The solute carrier 13 (SLC13) family comprises electrogenic sodium ion–coupled anion cotransporters, segregating into sodium ion–sulfate cotransporters (NaSs) and sodium ion–di- and–tricarboxylate cotransporters (NaDCs). NaS1 and NaDC1 regulate sulfate homeostasis and oxidative metabolism, respectively. From an overall view, both the NaDC1 and NaS1 form a homodimer, and each protomer consists of 11 TMDs. The rest TMDs form the core domain that is responsible for substrate recognition and conformational change to complete the transport cycle.

In this study, we determined the cryo–electron microscopy structures of human NaS1, capturing inward-facing and combined inward-facing/outward-facing conformations within a dimer both in apo and sulfate-bound states. For clarity, we have designated the NaS1 conformations as “IN/IN” for the inward-facing state, “IN/OUT” for the combined inward-facing/outward-facing states within a dimer, and “OUT/OUT” for the outward-facing conformation of NaDC1. Furthermore, the NaS1_IN/OUT conformations imply that each protomer within the dimer can independently execute the substrate transport cycle within SLC13 members. In this context, it is remarkable that TM1 to TM3 and TM9 of the dimerization domain maintain its structural integrity throughout the conformational change process, only minor changes of TM4, TM7, and TM8 are detected, emphasizing its role as a stable scaffold. However, the core domain, a pivotal player in the conformational transition, undergoes a notable movement. Furthermore, a more intricate conformational landscape emerges upon comparing the IN subunits of NaS1-IN/IN with the OUT subunits of NaS1_IN/OUT. This analysis reveals a dual-layered transition involving both horizontal and vertical displacements. Notably, the N and C halves within a given subunit undergo a remarkable conformational interchange, a dynamic interplay that mirrors the broader conformational shift of NaS1 during the transport cycle. Specifically, the binding pocket in the outward facing conformation of NaS1 could not accommodate the cholesterol molecule.

>MADYKDDDDKSGRMKFFSYILVYRRFLFVVFTVLVLLPLPIVLHTKEAECAYTLFVVATFWLTEALPLSVTALLPSLMLPMFGIMPSKKVASAYFKDFHLLLIGVICLATSIEKWNLHKRIALKMVMMVGVNPAWLTLGFMSSTAFLSMWLSNTSTAAMVMPIAEAVVQQIINAEAEVEATQMTYFNGSTNHGLEIDESVNGHEINERKEKTKPVPGYNNDTGKISSKVELEKNSGMRTKYRTKKGHVTRKLTCLCIAYSSTIGGLTTITGTSTNLIFAEYFNTRYPDCRCLNFGSWFTFSFPAALIILLLSWIWLQWLFLGFNFKEMFKCGKTKTVQQKACAEVIKQEYQKLGPIRYQEIVTLVLFIIMALLWFSRDPGFVPGWSALFSEYPGFATDSTVALLIGLLFFLIPAKTLTKTTPTGEIVAFDYSPLITWKEFQSFMPWDIAILVGGGFALADGCEESGLSKWIGNKLSPLGSLPAWLIILISSLMVTSLTEVASNPATITLFLPILSPLAEAIHVNPLYILIPSTLCTSFAFLLPVANPPNAIVFSYGHLKVIDMVKAGLGVNIVGVAVVMLGICTWIVPMFDLYTYPSWAPAMSNETMP[2x]> SMSPDKLVGDLHLFDNSVVFTAEELSCAPAEIIGRSCHGTSYKATLDNGYMLTVKWLKEGFAKSKKEFSREIKKLGSVRHPNLVPLRGYYWGPKEHERIMISDYADATSLSTYLSEFDERNLPPLSAGQRLNIAIDIARCLDYLHNERVIPHGNIKSSNVLIQNSTPSALVTDYSLHRLMTPIGMAEQVLNAGALGYSPPEFSSTSKPCPSLKSDVYAFGVILLELLTGKIAGEIICMNDGVVDLTDWVRMLD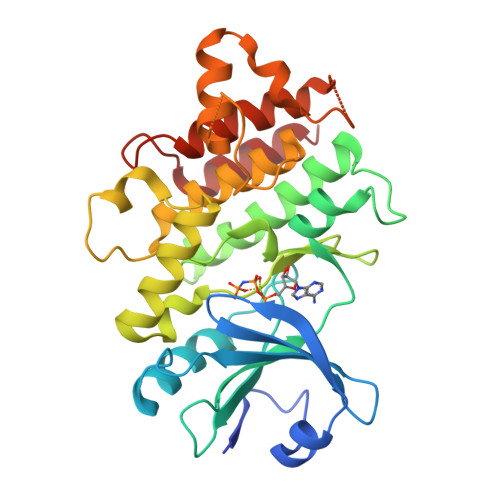LEERVSECYDRHITGVESSEGAPQALDGMLRIALRCIRSASERPEVRTVFEDLLSLSS>[2x]SSDKGKLSLQDVAELIRARACQRVVVMVGAGISTPSGIPDFRSPGSGLYSNLQQYDLPYPEAIFELPFFFHNPKPFFTLAKELYPGNYKPNVTHYFLRLLHDKGLLLRLYTQNIDGLERVSGIPASKLVEAHGTFASATCTVCQRPFPGEDIRADVMADRVPRCPVCTGVVKPDIVFFGEPLPQRFLLHVVDFPMADLLLILGTSLEVEPFASLTEAVRSSVPRLLINRDLVGPLAWHP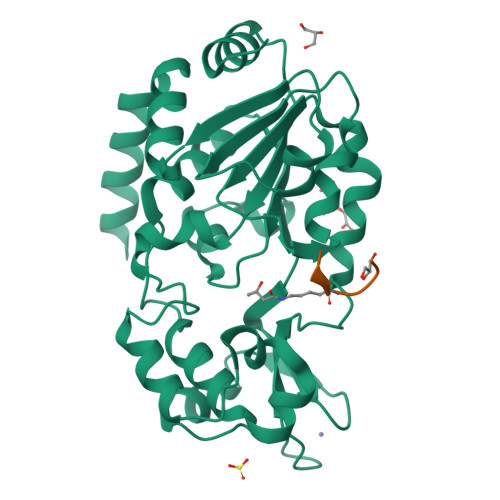RSRDVAQLGDVVHGVESLVELLGWTEEMRDLVQRETGKLDGPDK;>ARTXQTARKSTGGKA[2x]> GAMESEEPVFSLEQNRDDAMAALASTPTFQQTFINSISTQAMDLCKKYNLYPSVMIAQAALESNWGRSELGKAPNYNLFGIK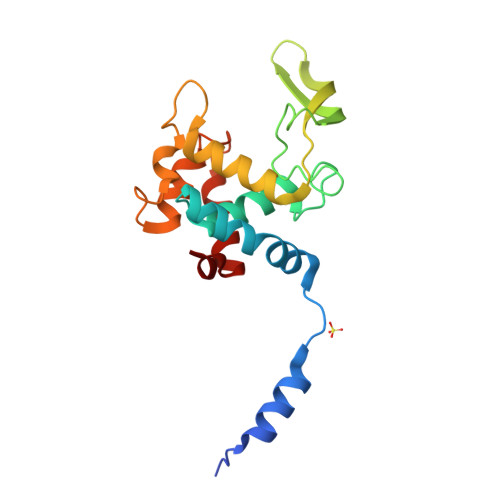GSYNGKSVTMKTWEYSDSKGWYQINANFAKYPSHKESLEDNAKKLRNGPSWDSSYYKGAWRENAKTYKDATAWLQGRYATDNTYASKLNTLISSYNLTQYD> ARAAFLFKTVGFGGLQNVPINDELSSHLLRAGNSPWQLTQFLDWISLGRGLATSALVPTAGSRYYQMSCLLSGTLQIPFRPNHRWGDIRFLRLVWSAPTLDGLVVAPPQVLAQPALQAQAD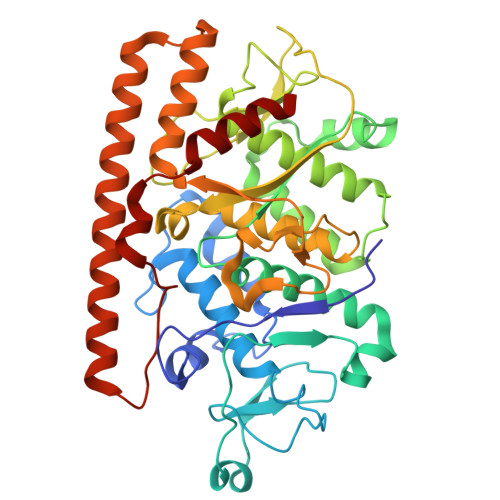RVYDCDDYPFLARDPRFKHRVYQQLSAVTLLNLTGFGPISYVRVDEDMWSGDVNQLLMNYFGHTFAEIAYTLCQASANRPWEYDGTYARMTQIVLSLFWLSYVGVIHQQNTYRTFYFQCNRRGDAAEVWILSCSLNHSAQIRPGNRSLFVMPTSPDWNMDVNLILSSTLTGCLCSGSQLPLIDNNSVPAVSRNIHGWTGRAGNQLHGFQVRRMVTEFCDRLRRDGVMTQAQQNQVEALADQTQQFKRDKLETWAREDDQYNQAHPNSTMFRTKPFTNAQWGRGNTGATSAAIAALI>MHRTYSLRNSRAPTASQLQNPPPPPSTTKGRFFGKGGLAYSFRRSAAGAFGPELSRKLSQLVKIEKNVLRSMELTANERRDAAKQLSIWGLENDDDVSDITDKLGVLIY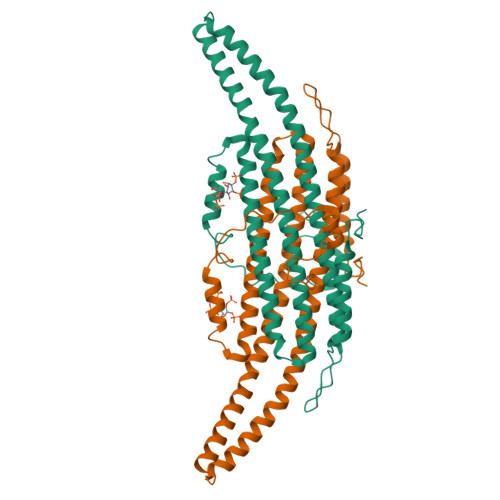EVSELDDQFIDRYDQYRLTLKSIRDIEGSVQPSRDRKDKITDKIAYLKYKDPQSPKIEVLEQELVRAEAESLVAEAQLSNITRSKLRAAFNYQFDSIIEHSEKIALIAGYGKALLELLDDSPVTPGETRPAYDGYEASKQIIIDAESALNEWTLDSAQVKPT[2x]>MADSDINIKTGTTDIGSNTTVKTGDLVTYDKENGMHKKVFYSFIDDKNHNKKLLVIRTKGTIAGQYRVYSEEGANKSGLAWPSAFKVQLQLPDNEVAQISDYYPRNSIDTKEYMSTLTYGFNSNVTGDDTGKIGGLIGANVSIGHTLRYVQPDFKTILESPTDKKVGWKVIFNNMVNQNWGPYDRDSWNPVYGNQLFMKTRNGSMKAADNFLDPNKASSLLSSGFSPDFATVITMDRKASKQQTNIDVIYERVRDDYQLHWTSTNWKGTNTKDKWTDRSSERYKIDWEKEEMTNGSSGSVTTLSGLSGEQGPSGDMTTEEDSATHIKFSKRDEDGRELAGATMELRDSSGKTISTWISDGHVKDFYLYPGKYTFVETAAPDGYEVATPIEFTVNEDGQVTVDGEATEGDAHTGGSHHHHHH[7x];>[7x]MADSDINIKTGTTDIGSNTTVKTGDLVTYDKENGMHKKVFYSFIDDKNHNKKLLVIRTKGTIAGQYRVYSEEGANKSGLAWPSAFKVQLQLPDNEVAQISDYYPRNSIDTKEYMSTLTYGFNSNVTGDDTGKIGGLIGANVSIGHTLRYVQPDFKTILESPTDKKVGWKVIFNNMVNQNWGPYDRDSWNPVYGNQLFMKTRNGSMKAADNFLDPNKASSLLSSGFSPDFATVITMDR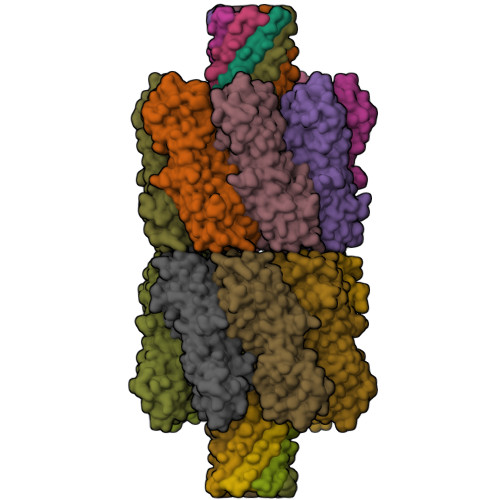KASKQQTNIDVIYERVRDDYQLHWTSTNWKGTNTKDKWTDRSSERYKIDWEKEEMTNGSSGSRGVPHIVMVDAYKRYKGGSHHHHHH A recently identified B. subtilis RRNPP member, RappLS20, is encoded by the Gram-positive B. subtilis conjugative plasmid pLS20. It lacks the conserved residues essential for phosphatase activity and has been shown to regulate the conjugation process. RappLS20 activates conjugation by acting as an antirepressor of RcopLS20 (22), which induces the formation of a DNA loop by binding to two closely located recognition sequences near the Pc, thereby inhibiting expression of the conjugation genes and plasmid transfer. The presence of the Phr*pLS20 peptide antagonizes the antirepressive action of RappLS20, reverting the system to its default state.

Crystals diffracting at 2.45 Å were obtained, and X-ray analyses revealed that the peptide-bound RappLS20 crystallized in a different space group with distinct cell parameters, consisting of four independent chains in the asymmetric unit. The electron density of the peptide was clearly observed in all chains. The peptide is oriented along the solenoid axis of the TPR domain, with its N-terminus bound in a closed pocket pointing towards the C-terminus of RappLS20. Recognition of the peptide by RappLS20 involves residues from helices H6, H8, H10, H12, H14 and H16. Phr*pLS20 adopts an extended conformation, with residues Q40 and K41 pointing in opposite directions with respect to the main chain, as do residues M43 and Y44. The superposition revealed that helices H6 and H7 (residues 129–166) of the TPR domain move inwards towards the center of the solenoid where the peptide binds, and upwards towards the C-terminus. We found that in the presence of the peptide, the NTDs move in a single direction and have a tendency to swing outward, away from the solenoid axis of the TPR. This movement can be observed to various degrees and was most pronounced for two of the four monomers (chains C and G) in the Phr*pLS20–RappLS20 structure, which each belong to the two different respective dimers. In the peptide-bound structure, two crystallographically independent tetramer configurations were found, which are formed through foot-2-foot interactions between two symmetry-related dimers. However, upon binding the signaling peptide, the NTDs shift outwards, facilitating the formation of the homotetramer, leading to a change of the interaction surface of the NTDs that is no longer available for interactions with RcopLS20.

>MLSKVKKVPSPYVGNLLNKWHDYIMQEKVHESIEKRTEIKQLLSQAEDNKDLVDYFILLDHRHSLCFDQEASMGDVVNMLSKGSHDLLINFYFELFAGDYEFFKKNYVKAISFYEKAEQKLSSIPNIEETKFAEFHYKIGVAYYEIDQHLVSVNKVTKARDIYKKSDMWNLEAIQCSLVVGINLYDMGRLDDADAYFRDALTEALDHGYDKPITKIYHNLGLVHWQKGSLELALHYFREAYSHEWLRDSPKGQQTVYMLSRVLYTMGQNEEAYHWYELGIEMARKFDDHEYKAKHDILYHLYEQPSIDEVKQSLAFLEERNLWPDVSKIAKGISELYEKKGDLVTSHEFLKRAFYAKEQIQRITEALGLEHHHHHH[4x];>[4x]MKKINGWIVVALLAVTTVGAAAAIQYTNNADSPGQFQVAQKGMY>[2x]MGTSLTDEELV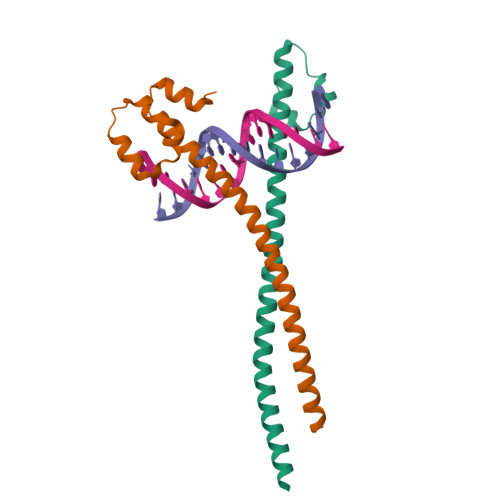TMSVRELNQHLRGLSKEEIVQLKQRRRTLKNRGYAASCRVKRVTQKEELEKQKAELQQEVEKLASENASMKLELDALRSKYEALQTFARTVAR;>GPHMAHLTRDELRAKALHIPFPVEKIINLPVVDFNEMMSKEQFNEAQLALIRDIRRRGKNKVAAQNCRKRKLENIVELEQDLDHLKDEKEKLLKEKGENDKSLHLLKKQLSTL[2x]> GPLGSPEFPGRLMKAGIDEAGKGCVIGPLVVAGVACSDEDRLRKLGVKDSKKLSQGRREELAEEIRKICRTEVLKVSPENLDERMAAKTINEILKECYAEIILRLKPEIAYVDSPDVIPERLSRELEEITGLRVVAEHKADEKYPLVAAASIIAKVER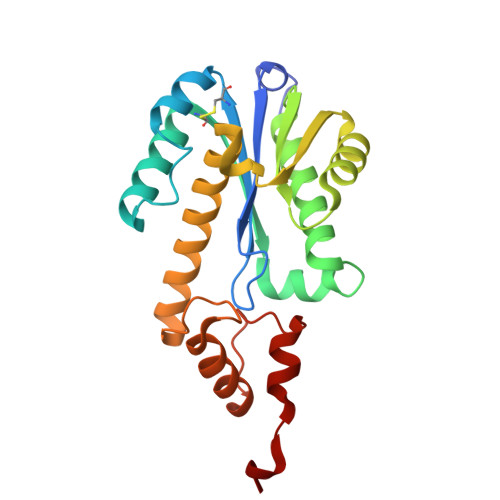EREIERLKEKFGDFGSGYASDPRTREVLKEWIASGRIPSCVRMRWKTVSNLRQKTLDDF> PQLPEVETIRRTLLPLIVGKTIEDVRIFWPNIIRHPRDS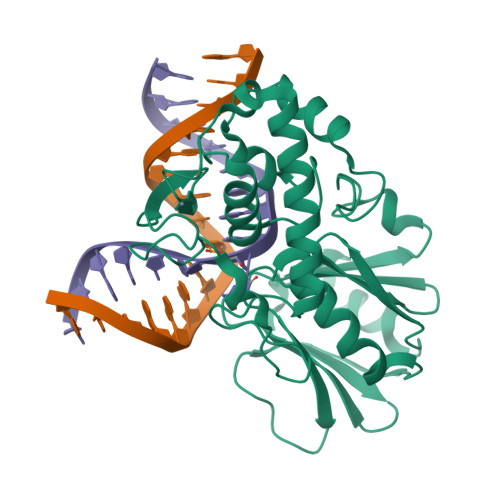EAFAARMIGQTVRGLERRGKFLKFLLDRDALISHLRMEGRYAVASALEPLEPHTHVVFCFTDGSELRYRDVRKFGTMHVYAKEEADRRPPLAELGPEPLSPAFSPAVLAERAVKTKRSVKALLLDCTVVAGFGNIYVDESLFRAGILPGRPAASLSSKEIERLHEEMVATIGEAVMKGGSTVRTYVNTQGEAGTFQHHLYVYGRQGNPCKRCGTPIEKTVVAGRGTHYCPRCQR> VVKQDLSDNQYIQKKPNEITSNELLLPLPNDKLLGDPKAPILMIEYASLTCYHCSLFHRNVFPKIKEKYIDTGKMLYIFRHFPLDYRGLKAAMLSHAYEKQEDYFNFNKAVFNSIDSWNYYNLSDLTLLQRIAALSNLKQDAFNQAINDKKIMDKIVNDKSLAINKLGITATPIFFIKLNDDKSYIEHNKVKHGGYKELKYFTNVIDKLYGKAIVK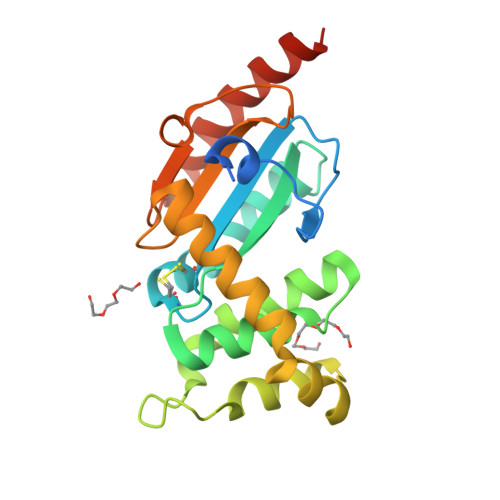LEHHHHHHHH> SEISRQEFQRRR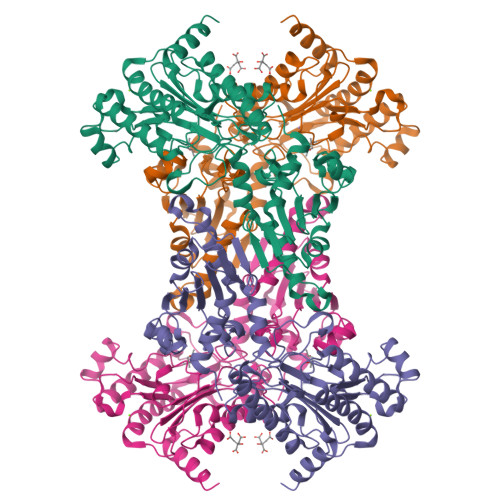QALVEQMQPGSAALIFAAPEVTRSADSEYPYRQNSDFWYFTGFNEPEAVLVLIKSDDTHNHSVLFNRVRDLTAEIWFGRRLGQDAAPEKLGVDRALAFSEINQQLYQLLNGLDVVYHAQGEYAYADVIVNSALEKLRKGSRQNLTAPATMIDWRPVVHEMRLFKSPEEIAVLRRAGEITAMAHTRAMEKCRPGMFEYHLEGEIHHEFNRHGARYPSYNTIVGSGENGCILHYTENECEMRDGDLVLIDAGCEYKGYAGDITRTFPVNGKFTQAQREIYDIVLESLETSLRLYRPGTSILEVTGEVVRIMVSGLVKLGILKGDVDELIAQNAHRPFFMAGLSHWLGLDVHDVGVYGQDRSRILEPGMVLTVEPGLYIAPDAEVPEQYRGIGIRIEDDIVITETGNENLTASVVKKPEEIEALMVAARKQ> CG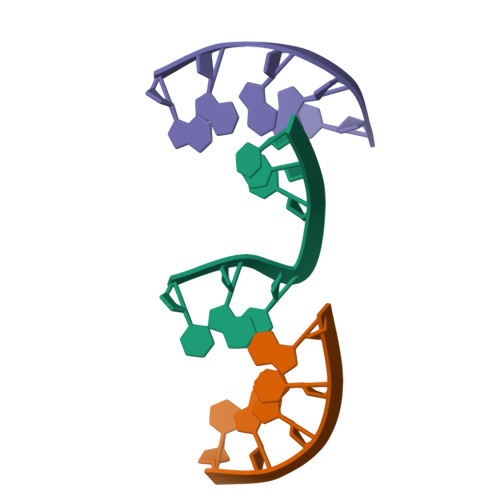ACG;> GGAGC;> CGTTCC> SEFF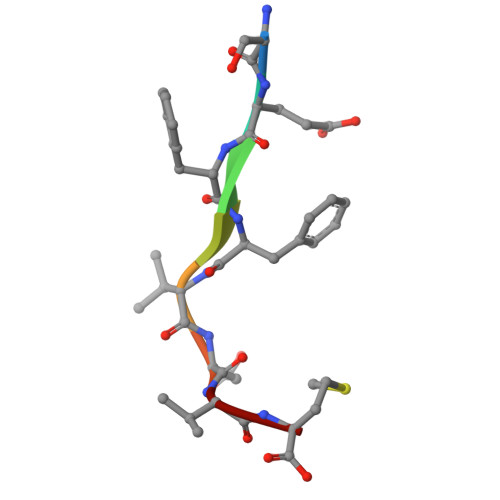VDVM>RKQISVRGLAGVENVTELKKNFNRHLHFTLVKDRNVATPRDYYFALAHTVRDHLVGRWIRTQQHYYEKDPKRIYYLSLEFYMGRTLQNTMVNLALENACDEATYQLGLDMEELEEIEEDAGLGNGGLGRLAACFLDSMATLGLAAYGYGIRYEFGIFNQKICGGWQMEEADDWLRYGNPWEKARPEFTLPVHFYGRVEHTSQGAKWVDTQVVLAMPYDTPVPGYRNNVVNTMRLWSAKAPNDFNLKDFNVGGYIQAVLDRNLAENISRVLYPNDNFFEGKELRLKQEYFVVAATLQDIIRRFKSSKFGCRDPVRTNFDAFPDKVAIQLNDTHPSLAIPELMRVLVDLERLDWDKAWEVTVKTCAYTNHTVIPEALERWPVHLLETLLPRHLQIIYEINQRFLNRVAAAFPGDVDRLRRMSLVEEGAVKRINMAHLCIAGSHAVNGVARIHSEILKKTIFKDFYELEPHKFQNKTNGITPRRWLVLCNPGLAEIIAERIGEEYISDLDQLRKLLSYVDDEAFIRDVAKVKQENKLKFAAYLEREYKVHINPNSLFDVQVKRIHEYKRQLLNCLHVITLYNRIKKEPNKFVVPRTVMIGGKAAPGYHMAKMIIKLITAIGDVVNHDPVVGDRLRVIFLENYRVSLAEKVIPAADLSEQISTAGTEASGTGNMKFMLNGALTIGTMDGANVEMAEEAGEEN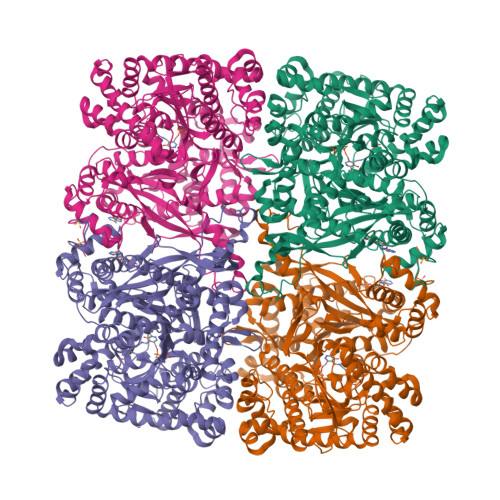FFIFGMRVEDVDRLDQRGYNAQEYYDRIPELRQIIEQLSSGFFSPKQPDLFKDIVNMLMHHDRFKVFADYEEYVKCQERVSALYKNPREWTRMVIRNIATSGKFSSDRTIAQYAREIWGVEPSRQRLPAP[4x]>[3x]MGSSHHHHHHSSGENLYFQGSAIATYNAHVYAALNLKSKVDTTFMAIGKTTAWTDETNPPEPDPNATGLTEVIGYKKLKTMSLCRPQRTGETPTLPTVSYGNKTWVLVPDAQAYTEG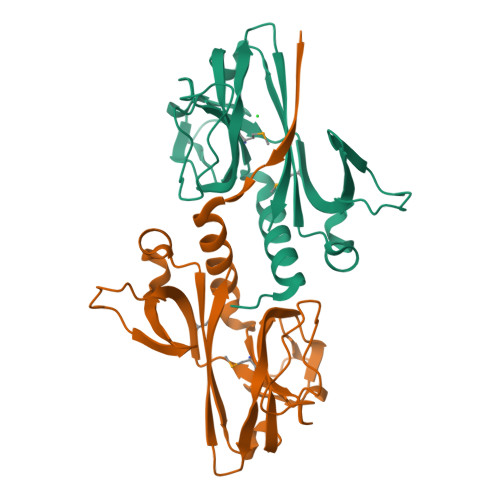AKWLYCEAEFVGDELPVGTYRQVGVFTDLAPKSGVTKPNLLPSEVANVGVLQFFENKQFQNRTPQVTARERFVAEL The 1,2-propanediol-utilizing microcompartment is assembled from seven different types of shell proteins, one of which is PduA. It is one of the more abundant components of the shell and intriguingly can form nanotubule-like structures when expressed on its own in the cytoplasm of Escherichia coli. The majority of shell proteins consist of a single BMC domain (Pfam 00936) in each subunit and assemble into hexamers. PduA has been shown to interact with the majority of the other shell proteins and, thus, could potentially act as a scaffold for the assembly of the microcompartment.

Overexpression of K26D or V51D mutant PduAs resulted in no higher order structures being observed by TEM in the bacterial cytoplasm despite the proteins being produced in quantities suitable for crystallization and structure determination (see results below). The lysine 26 mutant is the most important to study structurally because Lys-26 is conserved in all shell proteins and contributes significantly to the interface between 2-fold related hexamers in the native crystals. Two crystal forms were obtained for this mutant using commercially available screens. There is clear electron density for residues 4–89 in nine copies of the PduA subunit across the two crystal forms, and the C-terminal residues, including the additional 23 residues, are not seen in the electron density maps. In both crystal forms, the regularity of the tiling is lost in that the K26D PduA hexamer no longer has strict 6-fold symmetry, and the separation between hexamers is greater than in native PduA sheets (67.2 Å). In the first form, strips of hexamers are formed, and in the second, sheets with rather poor hexamer-hexamer interactions are seen. It is perhaps not surprising then that no structures are seen for the K26D mutant in the bacterial cytoplasm when PduA K26D is overexpressed. For one of these mutants (K26D), crystals were obtained, and these crystals reveal more fragile hexamer-hexamer tiling than in native PduA in one crystal form (type II) and only one-dimensional tiling in the other (type I). The mutation K26D has a profound influence on the conformation of the neighboring Arg-79, such that this region of the protein no longer adopts a single conformation in the crystal, resulting in breaking of the 6-fold symmetry axis of the hexamer. This results in the imperfect tiling of PduA molecules seen in the crystals and apparent lack of tiling at all in the bacterial cytoplasm.

>[6x]GSMQQEALGMVETKGLTAAIEAADAMVDSANVMLVGYEKIGSGLVTVIVRGDVGAVKAATDAGAAAARNVGEVKAVHVIPRPHTDVEKILPKGIRLVKDPAANKARKEAELAAATAEQ> MSLDLPEGHPLKTLYQENKEIMKDAEMLNLYAKTLATTK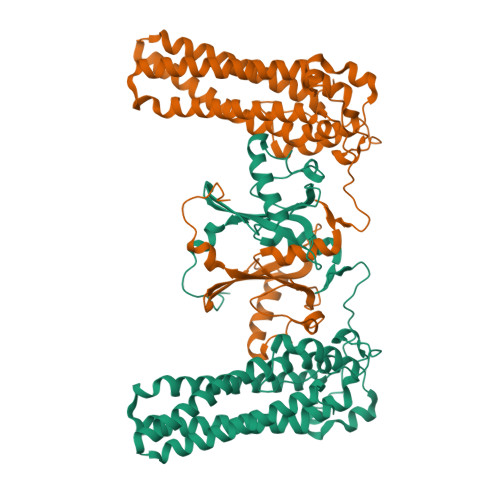DERMREEILGVLEEIVSSLRMVGFTHYNREEMLIFPYIERRGLTVIATVLWTKHDEIRAMIKQLAELLRKREEMPWEEFVEKFKAKAGEVAFALSDMVFRENNIFYPTLKALLSEGEWKAIKMQEDEIGYYKVKPPEWDPGEDVKPLHPWEINPELNVEQLLTLPKEVQQALRGQPLEFDKTQLKREEDIDLGTGYLNIEELKAIFEALPVDVTFIDKDDRVRFFSPGERIFTRTPSVLGRPVQLCHPPKSVYVVNKILKAFKEGRKKEATFWLRLREKYVYIKYVPLFNEKGEYIGTLEMTMDIAPYKKIEGEKRLLDWRDEGHHHHHH>[4x]QQELKQAEYQLSNARNLHNKLTNEMEACMRAVQT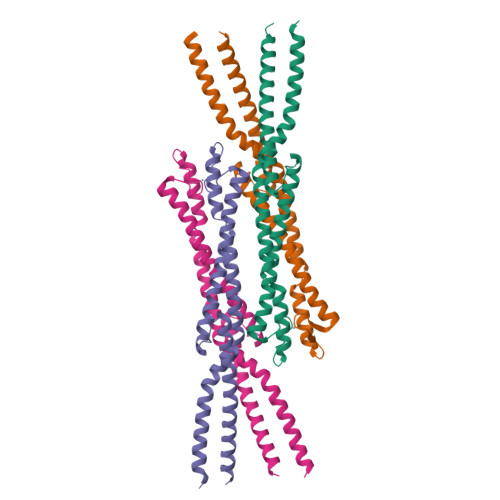AMKEARDLDSAPPVDEYITMLETDEKELAEVETALKLYDELKKHYSTIKDRALRFNKCYICDRDFTNQEAAKTRLLEKVAKRLGDEEKKELLEDQAAFMKSLDILRAVRVKYDTYQRLSSELPQLSREIDSETNRREDLVRRL>MTDDSAVESKQKKSKIRKGHWIPVVAGFLRKDGKILVGQRPENNSLAGQWEFPGGKIENGETPEEALARELNEELGIEAEVGELKLACTHSYGDVGILILFYEILYWKGEPRAK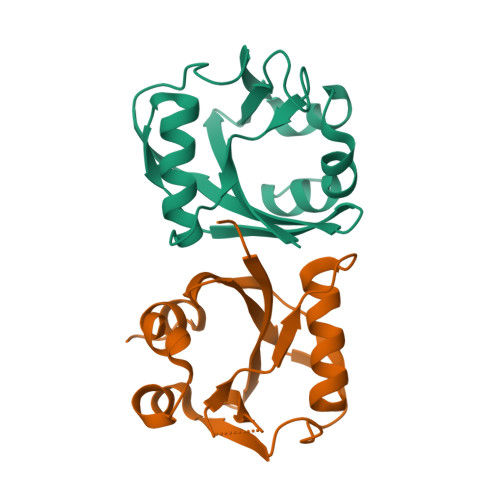HHMMLEWIHPEELKHRNIPEANRKILHKIYKALGLEWRK[2x]>[4x]MPVA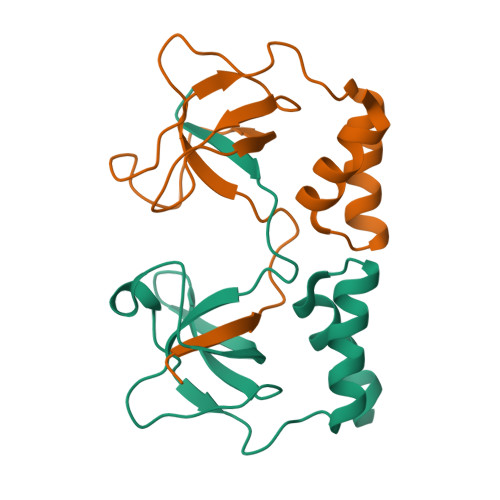HVALPVPLPRTFDYLLPEGMTVKAGCRVRVPFGKQQERIGIVVSVSDASELPLNELKAVVEVLDSEPVFTHSVWRLLLWAADYYHHPIGDVLFHALPILLR> DDLFASIGALWTW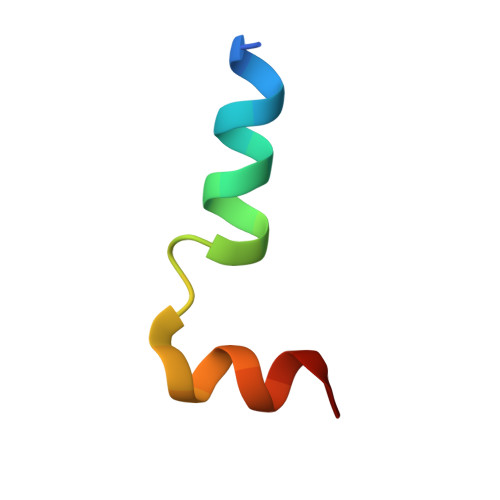AWRGPKARQELLKA> MARDEVRRILPADIKREVIVKDDKAETNPKWGFPPDKRP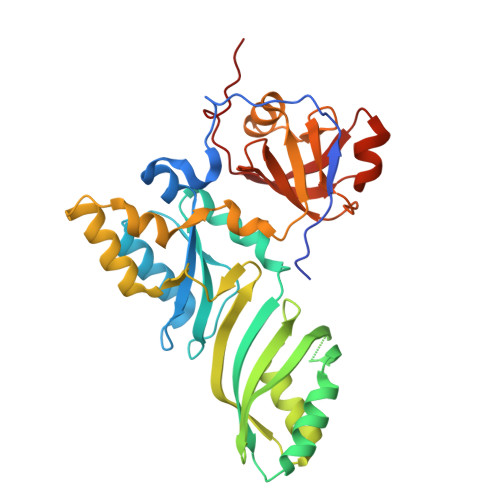IELHIQYGVINLDKPPGPTSHEVVAWIKRILNLEKAGHGGTLDPKVSGVLPVALERATRVVQALLPAGKEYVALMHLHGDVPEDKIRAVMKEFEGEIIQRPPLRSAVKRRLRTRKVYYIEILEIDGRDVLFRVGVEAGTYIRSLIHHIGLALGVGAHMAELRRTRSGPFKEDETLVTLHDLVDYYHFWKEDGIEEYIRKAIQPMEKAVEHLPKIWIKDSAVAAVAHGANLTVPGIVKLNAGIKKGDLVAIMTLKDELVALGKAMMSTQEMIERSKGIAVDVEKVFMPRDWYPKLW> MPELAVRTEFDYSSEIYKDAYSRINAIVIEGEQEAYSNYLQMAELLPEDKEELTRLAKMENRHKKGFQACGNNLQVNPDMPYAQEFFAGLHGNFQHAFSEGKVVTCLLIQALIIEAFAIAAYNIYIPVADDFARKITEGVVKDEYTHLNYGEEWLKANFATAKEELEQANKENLPLVWKMLNQVQGDAKVLGMEKEALVEDFMISYGEALSNIGFSTREIMRMSSYGLAGV

In 2010, Schirmer et al. identified two genes involved in fatty alk(a/e)ne biosynthesis in cyanobacteria: acyl-ACP reductase and aldehyde decarbonylase (renamed as aldehyde-deformylating oxygenase, ADO). The crystal structures of cADO revealed that cADO belongs to the non-heme dinuclear iron oxygenase family of enzymes exemplified by methane monoxygenase, type I ribonucleotide reductase, and ferritin. The di-iron center is contained within an antiparallel four-α-helix bundle, where two histidines and four carboxylates (aspartate or glutamate) supply the protein ligands to the metal ions. The C1-derived co-product of the cADO-catalyzed reaction is formate.

The variants of cADO-1593 from Synechococcus elongatus PCC7942 and cADO-sll0208 from Synechocystis sp. PCC6803 were constructed, overexpressed, purified and kinetically characterized. However, there is only one hydrogen bond between Asn123 and Tyr145 in 1593, and the corresponding residues forming the other hydrogen bond in sll0208 and PMT1231 are Gln49 and Phe150 in 1593. Thr159 of PMT1231 and the equivalent one (Thr146) of sll0208 are also involved in the hydrogen-bonding network close to the di-iron center. We have observed that 1593 is more active than sll0208 against n-hexadecanal, so Thr146, Leu148 and Tyr150 of sll0208 were respectively mutated into the counterparts of 1593 - Leu, Arg and Phe. Since PMT1231 is more active than sll0208 towards n-hexadecanal under our assay conditions (unpublished results), Asp49 and Asn123 of sll0208 were mutated into the corresponding residues of PMT1231 - His and His respectively. cat values of sll0208L148R and sll0208D49H/N123H were increased by 70.5 ± 5.3% and 65.9 ± 4.4% respectively, whereas those of sll0208D49H, sll0208N123H and sll0208T146L were significantly reduced. Firstly, the results of 1593L146T, 1593F150Y, sll0208T146L and sll0208L148R have clearly demonstrated that the side chains of the residues consisting of the oligopeptide (residues 144 to 150 for 1593) whose conformation changed in the absence of the di-iron center had important effects on cADO activity. Unexpectedly, the Y150F substitution of sll0208, in which the hydrogen bond between Tyr150 and Asp49 is removed, had negligible effect on the catalytic activity. The triple mutant 1593Q49H/F150Y/N123H showed higher activity than WT 1593, 1593Q49H/F150Y and 1593F150Y, and the double mutant sll0208D49H/N123H exhibited improved activity than WT sll0208, sll0208D49H and sll0208N123H. Thus, some synergistic effects were observed for 1593Q49H/F150Y/N123H and sll0208D49H/N123H, implying that these two hydrogen bonds are beneficial for cADO activity and the co-existence of two His in both hydrogen bonds is more important than the presence of only one His.> XFPP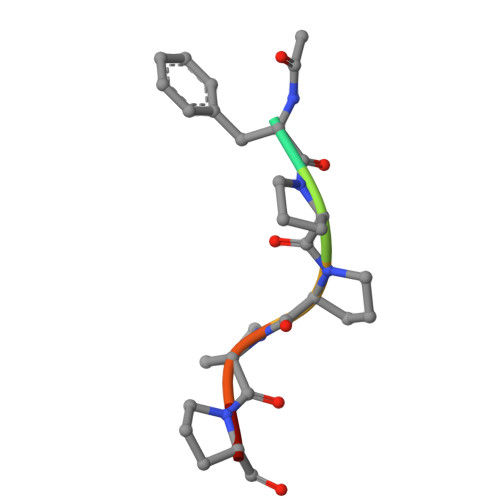PPT>HHNKVRTCWNEGRPALAGWLQLPGTLHAEALARLDYDAVVIDMQHSPIDFGQVAPMLIAIELGG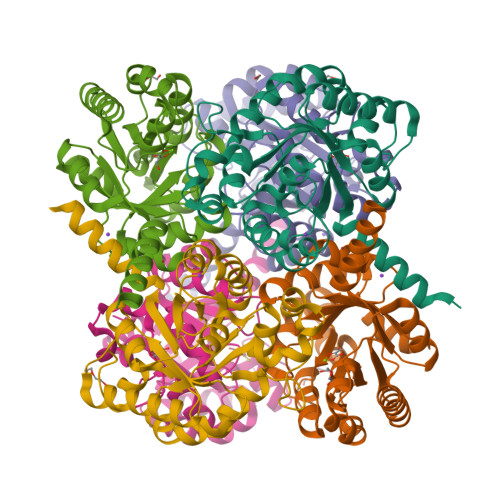AEPFVRTQVNDPSDIMKLLDAGAYGIIAPMVNTRAEAQTLASALHYSPRGLRSFGPRRPSLRYGSGYLAQASETVVGLAMIETREALANIDEILSVDGIDGVFIGPTDLALDLGHAPLVDTEEAEVVSAIAHVRERAHAAGKRVGIWCGSGGFARVKLAEGFDFVTAAPDLAMLSAAARQVIADARAL[2x]>GSSHHHHHHSSGENLYFQGHMTCPFADPAALYSRQDTTSGQSPLAAYEVDDSTGYLTSDVGGPIQDQTSLKAGIRGPTLLEDFMFRQKIQHFDHERVPERAVHARGAGAHGTFTSYADWSNITAASFLNATGKQTPVFVRFSTVAGSRGSADTARDVHGFATRFYTDEGNFDIVGNNIPVFFIQDAIQFPDLIHSVKPRPDNEIPQAATAHDSAWDFFSQQPSTMHTLFWAMSGHGIPRSYRHMDGFGVHTFRFVKDDGSSKLIKWHFKSRQGKASLVWEEAQVLSGKNADFHRQDLWDAIESGNGPEWDVCVQIVDESQAQAFGFDLLDPTKIIPEEYAPLTKLGLLKLDRNPTNYFAETEQVMFQPGHIVRGIDFTEDPLLQGRLFSYLDTQLNRNGGPNFEQLPINMPRVPIHNNNRDGAGQMFIHRNKYPYTPNTLNSGYPRQANQNAGRGFFTAPGRTASGALVREVSPTFNDHWSQPRLFFNSLTPVEQQFLVNAMRFEISLVKSEEVKKNVLTQLNRVSHDVAVRVAAAIGLGAPDADDTYYHNNKTAGVSIVGSGPLPTIKTLRVGILATTSESSALDQAAQLRTRLEKDGLVVTVVAETLREGVDQTYSTADATGFDGVVVVDGAAALFASTASSPLFPTGRPLQIFVDAYRWGKPVGVCGGKSSEVLDAADVPEDGDGVYSEESVDMFVEEFEKGLATFRFTDRFALDS[4x]

Catalases (hydrogen-peroxide:hydrogen-peroxide oxido­reductases; EC 1.11.1.6) are redox enzymes that are responsible for the dismutation of hydrogen peroxide into water and molecular oxygen. The structures reveal a homotetrameric enzyme in which each of the four active sites consists of a pentacoordinated iron protoporphyrin IX prosthetic group with a tyrosin­ate axial ligand. The heme is deeply buried inside the protein, with a complex network of channels providing access to the exterior. We have previously shown that in addition to catalase activity, the catalase from S. thermophilum (CATPO) possesses a promiscuous phenolic oxidase activity in the absence of hydrogen peroxide.

The mediation of the 3TR–CATPO interaction by water molecules in the plane of the inhibitor suggests a flexible binding site with the possibility of accommodating a variety of planar ligands of different sizes, suggesting that this could also be the site of phenolic substrate binding. The residues Pro158, His246, Gln293, Ile313, Ile314, Glu316, Leu321 and Val536 surround the 3TR binding pocket and are structurally homologous to the residues that bind NADPH in the mammalian catalases. However, the 3TR binding site for reversible inhibition has not been identified to date, although its noncompetitive nature would be consistent with a non-heme-centred mode of action. We therefore wondered whether this reversible inhibition could in fact be mediated via the oxidase substrate-binding site that we have identified. In this case, we would predict that catechol binding would protect the CATPO catalase activity against 3TR inhibition. We therefore carried out a competition assay at a constant concentration of 3TR (40 mM) that is sufficient to nearly totally inhibit the catalase activity and increasing amounts of catechol, and observed that the presence of catechol reduces 3TR inhibition in a dose-dependent manner. Interestingly, catechol itself inhibits the catalase activity, but in a much less potent fashion than 3TR. This suggests that, as proposed by others, the reversible inhibition by 3TR is mediated via an allosteric effect and that other molecules binding to this pocket will also have an inhibitory action. In this context it is interesting to note that the 3TR complex also shows a reduction in the number of ordered water molecules in the main channel when compared with the apo wild-type structure. In summary, based on our structural, mutation and kinetic data we propose that the pocket at the entrance to the lateral channel, occupied by the nicotinamide moiety of NADPH in mammalian catalases, is the site of both oxidase substrate and 3TR binding.> MGSNDYVNQMISQMTDLAKSLNVDVTELITSVTQALEALLEEYRREGRLTDQVEKMASSVALQLAAELLAQKALEEGHDKKQTTAKRNQISNSYSSEAMSHARAWAASRHSEEEAEKLAEELYKDMKESLKQRIDTEQVGSENLYFQ

Here we introduce Chroma, a generative model for proteins and protein complexes that can directly sample novel protein structures and sequences, and that can be conditioned to steer the generative process towards desired properties and functions. Given backbones from this diffusion process, the Chroma design network then generates sequence and side-chain conformations that are conditioned on the sampled backbone to yield a joint generative model for the sequences and structure of a protein complex. We sought to characterize the space of possible proteins parameterized by Chroma by generating a large number of unconditional samples of proteins and protein complexes (100,000 single-chain proteins and 20,000 complexes across two versions of the models, v.0 and v.1). The experimental characterization of 310 proteins shows that sampling from Chroma results in proteins that are highly expressed, fold and have favourable biophysical properties.

We reasoned that the best way to determine the plausibility of the protein space parameterized by Chroma was to draw independent samples from the model and test them experimentally. Our experimental validation shows that Chroma has learnt a sufficiently accurate distribution such that sampling from it results in proteins that express, fold, have favourable biophysical properties and conform to intended structures at non-trivial rates. The crystal structures of two designed proteins exhibit atomistic agreement with Chroma samples (a backbone root-mean-square deviation of around 1.0 Å). Moreover, the two designs with experimentally determined crystal structures demonstrate that a non-trivial fraction of this distribution should be expected to be atomistically accurate.>GAVKLNPDFSDAKENFYRVANWLVERWHFIMLNDTKRNTIYNAAIQKAVCLGSKSVLDIGAGTGILSMFAKKAGAHSVYACELSKTMYELACDVVAANKMEAGIKLLHTKSLDIEIPKHIPERVSLVVTETVDAGLFGEGIVESLIHAWEHLLLQPKTKGESANCEKYGKVIPASAVIFGMAVECAEIRRHHRVGIKDIAGIHLPTNVKFQSPAYSSVDTEETIEPYTTEKMSRVPGGYLALTECFEIMTVDFNNLQELKSLATKKPDKIGIPVIKEGILDAIMVWFVLQLDDEHSLSTSPSEETCWEQAVYPVQDLADYWIKPGDHVMMEVSCQDCYLRIQSISVLGLECEMDVAKSFTQNKDLLSLGNEAELCSALANLQTSKPDAVEQTCILESTEIALLNNIPYHEGFKMAMSKVLSSLTPEKLYQTMDTHCQNEMSSGTGQSNTVQNILEPFYVLDVSEGFSVLPVIAGTLGQVKPYSSVEKDQHRIALDLISEANHFPKETLEFWLRHVEDESAMLQRPKSDKLWSIIILDVIEP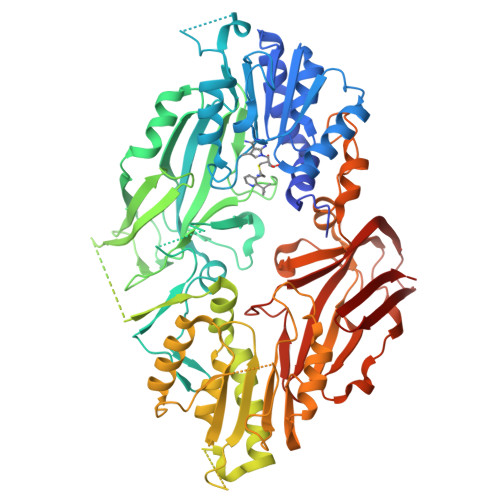SGLIQQEIMEKAAISRCLLQSGGKIFPQYVLMFGLLVESQTLLEENAVQGTERTLGLNIAPFINQFQVPIRVFLDLSSLPCIPLSKPVELLRLDLMTPYLNTSNREVKVYVCKSGRLTAIPFWYHMYLDEEIRLDTSSEASHWKQAAVVLDNPIQVEMGEELVLSIQHHKSNVSITVKQ[4x]N,N-dimethyl-L-valyl-L-leucyl-N-[(3S)-6-{(2S)-2-[([1,1'-biphenyl]-4-yl)methyl]-3-methoxy-5-oxo-2,5-dihydro-1H-pyrrol-1-yl}-6-oxo-1-phenylhexan-3-yl]-L-leucinamide 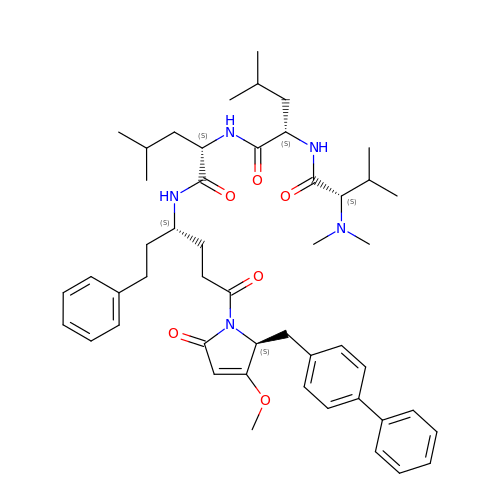| C49 H67 N5 O6 | JLQMIAJVDKBAJR-BFALPNPBSA-N> MRLLLVEDHVPLADELMASLTRQGYAVDWLADGRDAAVQGASEPYDLIILDL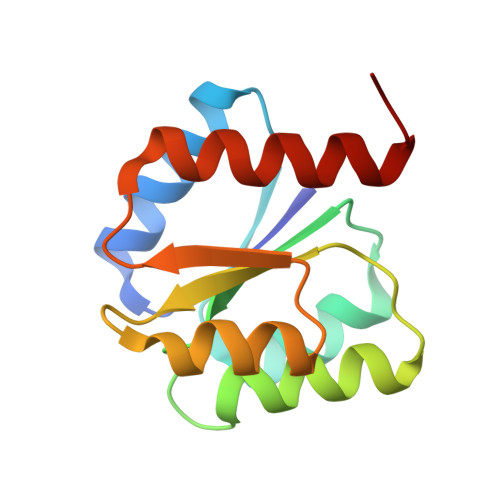GLPGRPGLEILQEWRGLGLATPVLILTARGSWAERIDGLKAGADDYLTKPFHPEELALRIQALLRRAHGLA> MAHHHHHHMETKTQYVPYKVKDISLAEWGRKEIELAEAEMPGLMAIREEYGPQQPLKGARIAGCLHMTIQTAVLIETLVALGADVTWSSCNIFSTQDHAAAAIAAAGIPV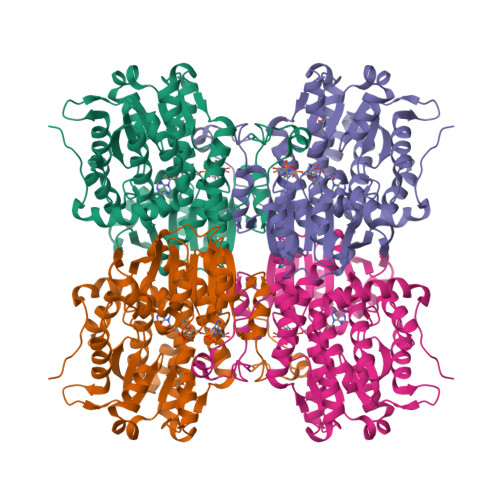YAWKGMNEEEFDWCIEQTLFFGEDRQPLNMILDDGGDLTNMVFDKYPELTKDIKGLSEETTTGVHRLYERMQNGTLVMPAINVNDSVTKSKFDNKYGCRESAVDAIRRATDVMLAGKRVVVCGFGDVGKGTAASFRGAGSIVTVTEIDPICALQAAMEGYEVKQLDTVVDNADIIITTTGNFGIVRGEHFEKMKDKTIVCNIGHFDNEIDMAWLNKNHGATKVEIKPQVDKYNVNGNDIIILAEGRLVNLGCATGHPSFVMSNSFSNQTLAQIELWVHSDKYENKVYTLPKHLDEKVAALHLKKLGVELETLSEEQAKYIGVTVDGPFKPDYYRY> MDPIINGNSANVYLTDSYLKGVISFSECNALGSYIFNGPYLKNDYTNLISRQNPLIEHMNLKKLNITQSLISKYHKGEIKLEEPTYFQSLLMTYKSMTSSEQIATTNLLKKIIRRAIEISDVKVYAILNKLGLKEKDKIKSNNGQDEDNSVITTIIKDDILSAVKDNQSHLKADKNHSTKQKDTIKTTLLKKLMCSMQHPPSWLIHWFNLYTKLNNILTQYRSNEVKNHGFTLIDNQTLSGFQFILNQYGCIVYHKELKRITVTTYNQFLTWKDISLSRLNVCLITWISNCLNTLNKSLGLRCGFNNVILTQLFLYGDCILKLFHNEGFYIIKEVEGFIMSLILNITEEDQFRKRFYNSMLNNITDAANKAQKNLLSRVCHTLLDKTVSDNIINGRWIILLSKFLKLIKLAGDNNLNNLSELYFLFRIFGHPMVDERQAMDAVKINCNETKFYLLSSLSMLRGAFIYRIIKGFVNNYNRWPTLRNAIVLPLRWLTYYKLNTYPSLLELTERDLIVLSGLRFYREFRLPKKVDLEMIINDKAISPPKNLIWTSFPRNYMPSHIQNYIEHEKLKFSESDKSRRVLEYYLRDNKFNECDLYNCVVNQSYLNNPNHVVSLTGKERELSVGRMFAMQPGMFRQVQILAEKMIAENILQFFPESLTRYGDLELQKILELKAGISNKSNRYNDNYNNYISKCSIITDLSKFNQAFRYETSCICSDVLDELHGVQSLFSWLHLTIPHVTIICTYRHAPPYIGDHIVDLNNVDEQSGLYRYHMGGIEGWCQKLWTIEAISLLDLISLKGKFSITALINGDNQSIDISKPIRLMEGQTHAQADYLLALNSLKLLYKEYAGIGHKLKGTETYISRDMQFMSKTIQHNGVYYPASIKKVLRVGPWINTILDDFKVSLESIGSLTQELEYRGESLLCSLIFRNVWLYNQIALQLKNHALCNNKLYLDILKVLKHLKTFFNLDNIDTALTLYMNLPMLFGGGDPNLLYRSFYRRTPDFLTEAIVHSVFILSYYTNHDLKDKLQDLSDDRLNKFLTCIITFDKNPNAEFVTLMRDPQALGSERQAKITSEINRLAVTEVLSTAPNKIFSKSAQHYTTTEIDLNDIMQNIEPTYPHGLRVVYESLPFYKAEKIVNLISGTKSITNILEKTSAIDLTDIDRATEMMRKNITLLIRILPLDCNRDKREILSMENLSITELSKYVRERSWSLSNIVGVTSPSIMYTMDIKYTTSTISSGIIIEKYNVNSLTRGERGPTKPWVGSSTQEKKTMPVYNRQVLTKKQRDQIDLLAKLDWVYASIDNKDEFMEELSIGTLGLTYEKAKKLFPQYLSVNYLHRLTVSSRPCEFPASIPAYRTTNYHFDTSPINRILTEKYGDEDIDIVFQNCISFGLSLMSVVEQFTNVCPNRIILIPKLNEIHLMKPPIFTGDVDIHKLKQVIQKQHMFLPDKISLTQYVELFLSNKTLKSGSHVNSNLILAHKISDYFHNTYILSTNLAGHWILIIQLMKDSKGIFEKDWGEGYITDHMFINLKVFFNAYKTYLLCFHKGYGKAKLECDMNTSDLLCVLELIDSSYWKSMSKVFLEQKVIKYILSQDASLHRVKGCHSFKLWFLKRLNVAEFTVCPWVVNIDYHPTHMKAILTYIDLVRMGLINIDRIHIKNKHKFNDEFYTSNLFYINYNFSDNTHLLTKHIRIANSELENNYNKLYHPTPETLENILANPIK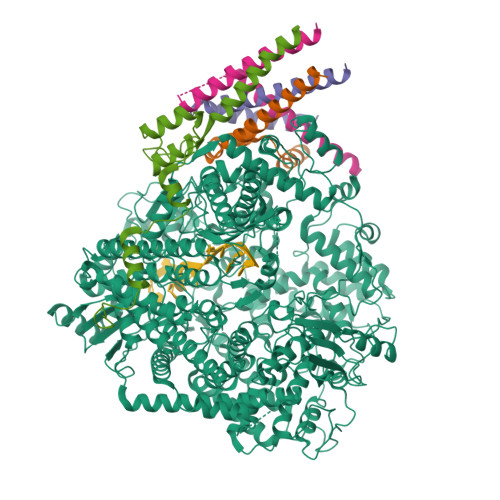SNDKKTLNDYCIGKNVDSIMLPLLSNKKLIKSSAMIRTNYSKQDLYNLFPMVVIDRIIDHSGNTAKSNQLYTTTSHQISLVHNSTSLYCMLPWHHINRFNFVFSSTGCKISIEYILKDLKIKDPNCIAFIGEGAGNLLLRTVVELHPDIRYIYRSLKDCNDHSLPIEFLRLYNGHINIDYGENLTIPATDATNNIHWSYLHIKFAEPISLFVCDAELSVTVNWSKIIIEWSKHVRKCKYCSSVNKCMLIVKYHAQDDIDFKLDNITILKTYVCLGSKLKGSEVYLVLTIGPANIFPVFNVVQNAKLILSRTKNFIMPKKADKESIDANIKSLIPFLCYPITKKGINTALSKLKSVVSGDILSYSIAGRNEVFSNKLINHKHMNILKWFNHVLNFRSTELNYNHLYMVESTYPYLSELLNSLTTNELKKLIKITGSLLYNFHNE;>[4x]MEKFAPEFHGEDANNRATKFLESIKGKFTSPKDPKKKDSIISVNSIDIEVTKESPITSNSTIINPTNETDDTAGNKPNYQRKPLVSFKEDPTPSDNPFSKLYKETIETFDNNEEESSYSYEEINDQTNDNITARLDRIDEKLSEILGMLHTLVVASAGPTSARDGIRDAMVGLREEMIEKIRTEALMTNDRLEAMARLRNEESEKMAKDTSDEVSLNPTSEKLNNLLEGNDSDNDLSLEDF>[4x]MHHHHHHHHHGGPISKILVANRSEIAIRVFRAANELGIKTVAIWAEEDKLALHRFKADESYQVGRGPHLARDLGPIESYLSIDEVIRVAKLSGADAIHPGYGLLSESPEFVDACNKAGIIFIGPKADTMRQLGNKVAARNLAISVGVPVVPATEPLPDDMAEVAKMAAAIGYPVMLKASWGGGGRGMRVIRSEADLAKEVTEAKREAMAAFGKDEVYLEKLVERARHVESQILGDTHGNVVHLFERDCSVQRRNQKVVERAPAPYLSEAQRQELAAYSLKIAGATNYIGAGTVEYLMDADTGKFYFIEVNPRIQVEHTVTEVVTGIDIVKAQIHILDGAAIGTPQSGVPNQEDIRLNGHALQCRVTTEDPEHNFIPDYGRITAYRSASGFGIRLDGGTSYSGAIITRYYDPLLVKVTAWAPNPLEAISRMDRALREFRIRGVATNLTFLEAIIGHPKFRDNSYTTRFIDTTPELFQQVKRQDRATKLLTYLADVTVNGHPEAKDRPKPLEN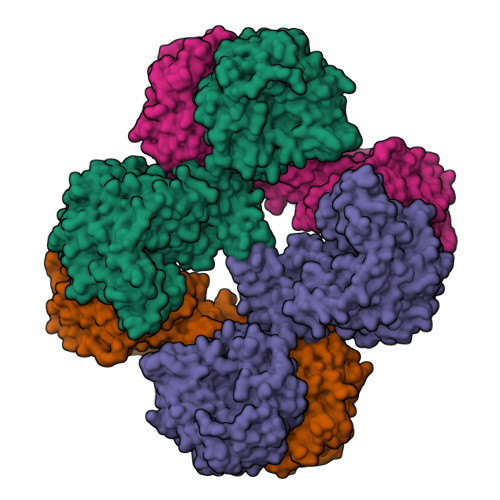AARPVVPYANGNGVKDGTKQLLDTLGPKKFGEWMRNEKRVLLTDTTMRDGHQSLLATRMRTYDIARIAGTYSHALPNLLSLECWGGATFDVSMRFLTEDPWERLALIREGAPNLLLQMLLRGANGVGYTNYPDNVVKYFVRQAAKGGIDLFRVFDCLNWVENMRVSMDAIAEENKLCEAAICYTGDILNSARPKYDLKYYTNLAVELEKAGAHIIAVKDMAGLLKPAAAKVLFKALREATGLPIHFHTHDTSGIAAATVLAAVEAGVDAVDAAMDALSGNTSQPCLGSIVEALSGSERDPGLDPAWIRRISFYWEAVRNQYAAFESDLKGPASEVYLHEMPGGQFTNLKEQARSLGLETRWHQVAQAYADANQMFGDIVKVAPSSKVVGDMALMMVSQDLTVADVVSPDREVSFPESVVSMLKGDLGQPPSGWPEALQKKALKGEKPYTVRPGSLLKEADLDAERKVIEKKLEREVSDFEFASYLMYPKVFTDFALASDTYGPVSVLPTPAYFYGLADGEELFADIEKGKTLVIVNQAVSATDSQGMVTVFFELNGQPRRIKVPDRAHGATGAAVRRKAEPGNAAHVGAPMPGVISRVFVSSGQAVNAGDVLVSIEAMKMETAIHAEKDGTIAEVLVKAGDQIDAKDLLAVYGG> SMKLVKFRKGDSVGLRLAGGNDVGIFVAGVLEDSPAAKEGLEEGDQILRVNNVDFTNIIREEAVLFLLDLPKGEEVTILAQKKKDVYRRIVESDVGDSFYIRTHFEYEKESPYGLSFNKGEVFRVVDTLYNGKLGSWLAIRIGKNHKEVERGIIPNKNRAEQLASVQYTLPKTAGGDRADFWRFRGLRSSKRNLRKSREDLSAQPVQTKFPAYERVVLREAGFLRPVTIFGPIADVAREKLAREEPDIYQIAKSEPRDAGTDQRSSGIIRLHTIKQIIDQDKHALLDVTPNAVDRLNYAQWYPIVVFLNPDSKQ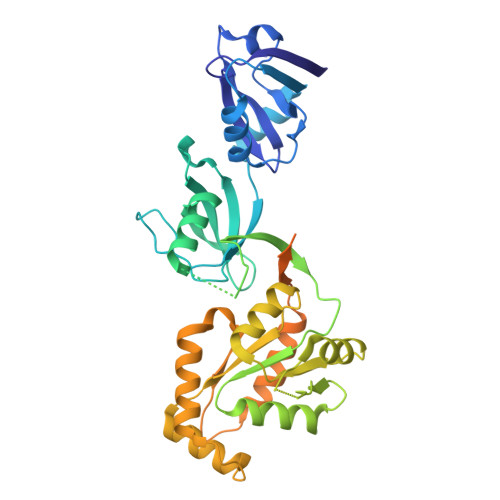GVKTMRMRLCPESRKSARKLYERSHKLRKNNHHLFTTTINLNSMNDGWYGALKEAIQQQQNQLVWVSEGKADGATSDDLDLHDDRLSYLSAPGSEYSMYSTDSRHTSDYEDTDTEGGAYTDQELDETLNDEVGTPPESAITRSSEPVREDSSGM N-[(4'-IODOBIPHENYL-4-YL)SULFONYL]-D-TRYPTOPHAN | 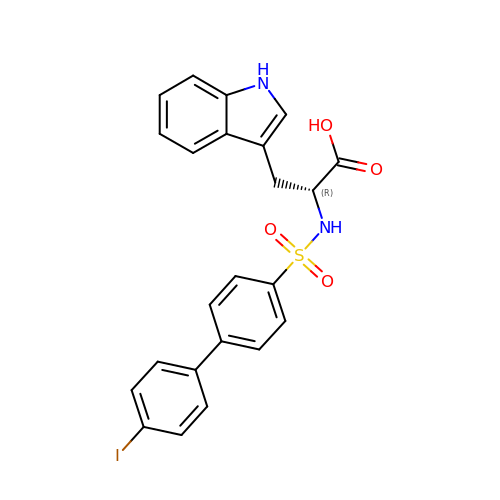C23 H19 I N2 O4 S | BLBDKMAMVNXYIE-JOCHJYFZSA-N> SVIRWCTISSPEEKKCNNLRDLTQQERISLTCVQKATYLDCIKAIANNEADAISLD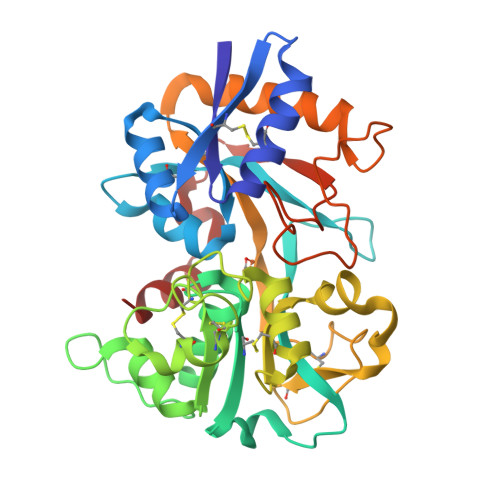GGQAFEAGLAPYKLKPIAAEVYEHTEGSTTSYYAVAVVKKGTEFTVNDLQGKTSCHTGLGRSAGWNIPIGTLLHRGAIEWEGIESGSVEQAVAKFFSASCVPGATIEQKLCRQCKGDPKTKCARNAPYSGYSGAFHCLKDGKGDVAFVKHTTVNENAPDQKDEYELLCLDGSRQPVDNYKTCNWARVAAHAVVARDDNKVEDIWSFLSKAQSDFGVDTKSDFHLFGPPGKKDPVLKDLLFKDSAIMLKRVPSLMDSQLYLGFEYYSAIQSMR> MAIIETTTPTEEEAK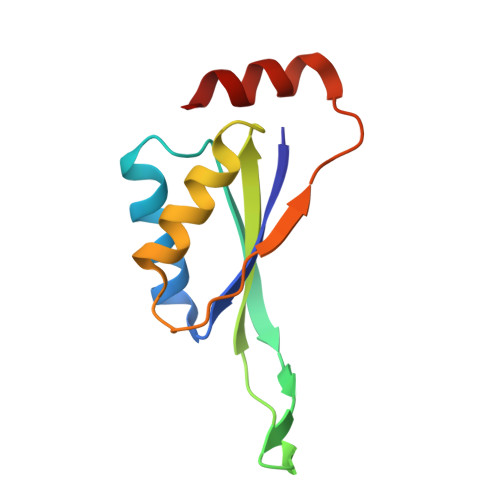AIAKKLLENRLIAEAIITPALTKIYRENGEIKSETVTRVTLYTEEENVPKAVTYIKAIHPDPIPPIIVITPTDANPAYKGWVAFET>[2x]AKHLFTSESVSEGHPDKIADQISDAVLDAILEQDPKARVACETYVKTGMVLVGGEITTSAWVDIEEITRNTVREIGYVHSDMGFDANSCAVLSAIGKQSPDINQGVDRADPLEQGAGDQGLMFGYATNETDVLMPAPITYAHRLVQRQA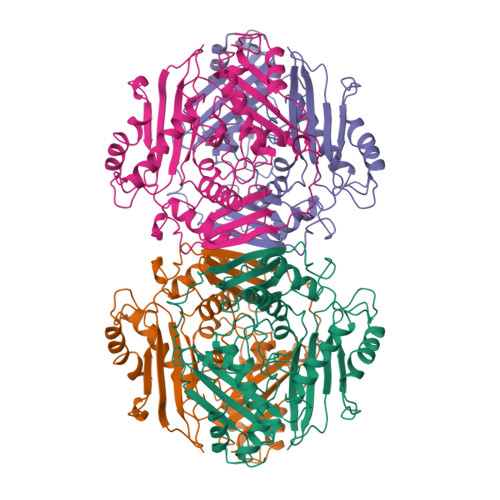EVRKNGTLPWLRPDAKSQVTFQYDDGKIVGIDAVVLSTQHSEEIDQKSLQEAVMEEIIKPILPAEWLTSATKFFINPTGRFVIGGPMGDCGLTGRKIIVDTYGGMARHGGGAFSGKDPSKVDRSAAYAARYVAKNIVAAGLADRCEIQVSYAIGVAEPTSIMVETFGTEKVPSEQLTLLVREFFDLRPYGLIQMLDLLHPIYKETAAYGHFGREHFPWEKTDKAQLLRDAAGLK> MKELNDLEKKYNAHIGVYALDTKSGKEVKFNSDKRFAYASTSKAINSAILLEQVPYNKLNKKVHINKDDIVAYSPILEKYVGKDITLKALIEASMTYSDNTANNKIIKEIGGIKKVKQRLKELGDKVTNPVRYDIELQYYSPKSKKDTS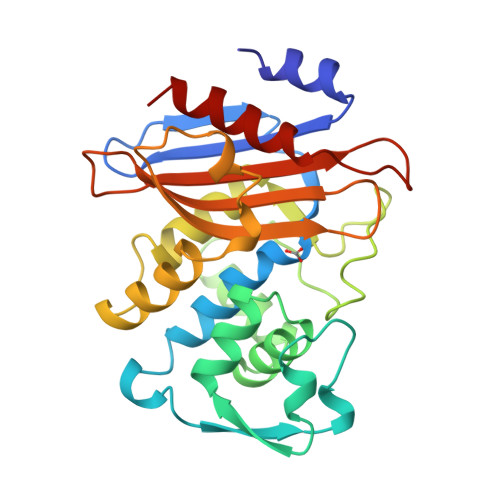TPAAFGKTLNKLIANGKLSKENKKFLLDLMLNNKSGDTLIKDGVPKDYKVADKSGQAITYASRNDVAFVYPKGQSEPIVLVIFTNKDNKSDKPNDKLISETAKSVMKEF> MRVSHEQFRAALQLVVSPGDPREYLANFIKIGEGSTGIVCIATEKHTGKQVAVKKMDLRKQQRRELLFNEVVIMRDYHHDNVVDMYSSYLVGDELWVVMEFLEGGALTDIVTHTRMNEEQIATVCLSVLRALSYLH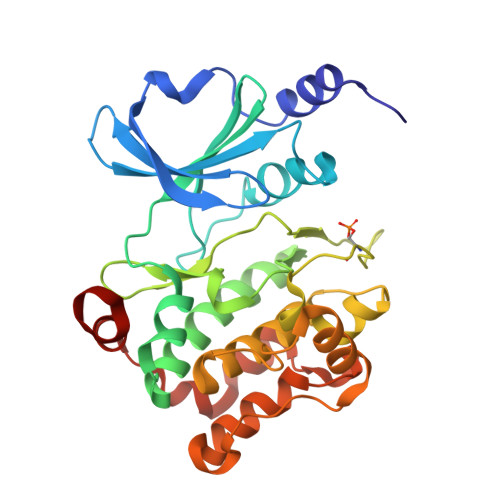NQGVIHRDIKSDSILLTSDGRIKLSDFGFCAQVSKEVPKRKSLVGTPYWMAPEVISRLPYGTEVDIWSLGIMVIEMIDGEPPYFNEPPLQAMRRIRDSLPPRVKDLHKVSSVLRGFLDLMLVREPSQRATAQELLGHPFLKLAGPPSCIVPLMRQYRHH> MKITDLELHAVGIPRHTGFVNKHVIVKIHTDEGLTGIGEMSDFSHLPLYSVDLHDLKQGLLS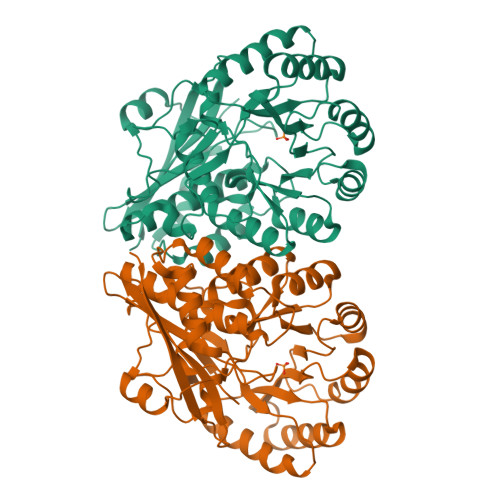ILLGQNPFDLMKINKELTDNFPETMYYYEKGSFIRNGIDNALHDLCAKYLDISVSDFLGGRVKEKIKVCYPIFRHRFSEEVESNLDVVRQKLEQGFDVFRLYVGKNLDADEEFLSRVKEEFGSRVRIKSYDFSHLLNWKDAHRAIKRLTKYDLGLEMIESPAPRNDFDGLYQLRLKTDYPISEHVWSFKQQQEMIKKDAIDIFNISPVFIGGLTSAKKAAYAAEVASKDVVLGTTQELSVGTAAMAHLGCSLTNINHTSDPTGPELYVGDVVKNRVTYKDGYLYAPDRSVKGLGIELDESLLAKYQVPDLSWDNVTVHQLQDRTADTKS>[2x]SMLAELITSYRKSAAIYAFVDTGLSIHFRNGAYVDIDELSRQCGIDYSRLDRLCDFLI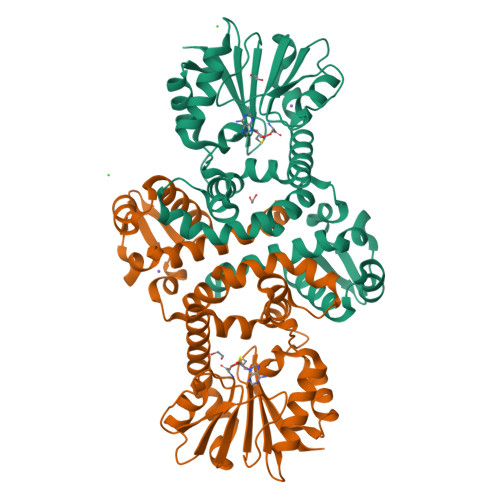EIGILVNHGHKVTLSEECSALADPESMESLMVKLELSPDYWNAWSMYPRSLLENDGKPAFEITHGKSFFEHLASNKLLKSNFDSLMSKVSDKIIEKLLDIYDFGQYNRILDIGGGEGSLLVKMSEKVKGKHYAVLDRYDEIPVLENIDFINGDFLKVIPSGYDLYILKDVIHDWSDNNAILILENCRKAMDNGSAVLLISMMKKPQSKMVIYFDILMDVLFSGKERYLTEFERLANQAGLVIQDVKDIDESYSIIQLGIK> MDGSGEQPRGGGPTSSEQIMKTGALLLQGFIQDRAGRMGGEAPELALDPVPQDASTKKLSESLKRIGDELDSNMELQRMIAAVDTDSPREVFFRVAADMFSDGNFNWGRVVALFYFASKLVLKALSTKVPELIRTIMGWTLDFLRERLLGWIQDQGGWDGLLSYFGSS;> DMRPEIWIAQELRRIGDEFN

The intrinsic pathway to apoptosis is regulated by interactions between members of three factions of the Bcl-2 protein family: the BH3-only proteins such as Bim and Bid, which initiate the process, the essential effectors Bax and Bak, and the prosurvival members, which oppose the action of both other factions. Unlike Bak, which is constitutively anchored in the mitochondrial outer membrane (MOM) via its C-terminal segment, Bax is largely cytosolic in healthy cells and accumulates at the MOM only upon a death signal. Core/latch dimers of Bax and Bak form on treatment of the monomeric proteins with certain BH3 peptides and CHAPS, and Bax and Bak core domains form symmetric homodimers, supporting that unlatching the core domain is a necessary step to Bax and Bak oligomerisation and permeabilisation of the MOM. Bim and Bid are both potent direct activators of Bax, but Bim is less dependent on interactions via its ‘h0' residues than is Bid.

We previously showed that mini-BH3 motifs, 20-mers spanning residues ‘h0'–‘h4', sufficed to trigger dissociation of BaxΔC into core and latch domains. To confirm that the N- and C-terminal segments of the longer peptides did not influence the peptides' interaction with Bax, we crystallised both BimBH3mini and BidBH3mini with BaxΔC26. These structures are essentially identical to that reported above and to BidBH3:BaxΔC21 (PDB 4BD27), except to note that in the case of the BimBH3mini complex, no clear density is evident for F159 (the ‘h4' residue). Note also that the conformation of F30 in the BimBH3mini:BaxΔC26 complex resembles that found in all of the BidBH3 complexes with Bax that we have studied, further suggesting that the altered orientation of this residue in the BimBH3:BaxΔC26 structure stems from the different crystallisation conditions. The BH3mini:BaxΔC26 complexes contain a cavity between helices α1, α2, α5 and α8 (shaped with the side chains of residues 26, 30, 60, 63, 66, 67, 110, 111, 114, 115, 158 and 161) as observed also in the BidBH3:BaxΔC21 complex but not in the apo BaxΔC21 core/latch dimer. F30 is among those residues whose backbone amide resonance is grossly affected by titration of the BaxBH3 peptide into BaxΔC21.37 We interpret the presence of cavities within the core of Bax when bound to an activator BH3 peptide as a sign of instability of the complex, pre-empting the release of the Bax latch domain (α6–α8) as required for the core domains (α2–α5) to dimerise. Note that we have calculated the cavity using the structure of the BimBH3mini:BaxΔC26 complex, because the anomalous conformation of F30 in the BimBH3:BaxΔC26 described above obscures the effect.>MCKDKNEKKNYEHVNANEKNGYLASEKNELTKNKVEEHTYDYDYVVIGGGPGGMASAKEAAAHGARVLLFDYVKPSSQGTKWGIGGTCVNVGCVPKKLMHYAGHMGSIFKLDSKAYGWKFDNLKHDWKKLVTTVQSHIRSLNFSYMTGLRSSKVKYINGLAKLKDKNTVSYYLKGDLSKEETVTGKYILIATGCRPHIPDDVEGAKELSITSDDIFSLKKDPGKTLVVGASYVALECSGFLNSLGYDVTVAVRSIVLRGFDQQCAVKVKLYMEEQGVMFKNGILPKKLTKMDDKILVEFSDKTSELYDTVLYAIGRKGDIDGLNLESLNMNVNKSNNKIIADHLSCTNIPSIFAVGDVAENVPELAPVAIKAGEILARRLFKDSDEIMDYSYIPTSIYTPIEYGACGYSEEKAYELYGKSNVEVFLQEFNNLEISAVHRQKHIRAQKDEYDLDVSSTCLAKLVCLKNEDNRVIGFHYVGPNAGEVTQGMALALRLKVKKKDFDNCIGIHPTDAESFMNLFVTISSGLSYAAKGGSGGGKCG[4x];>RGSHHHHHHGSVKIVTSQAEFDSIISQNELVIVDFFAEWCGPSKRIAPFYEECSK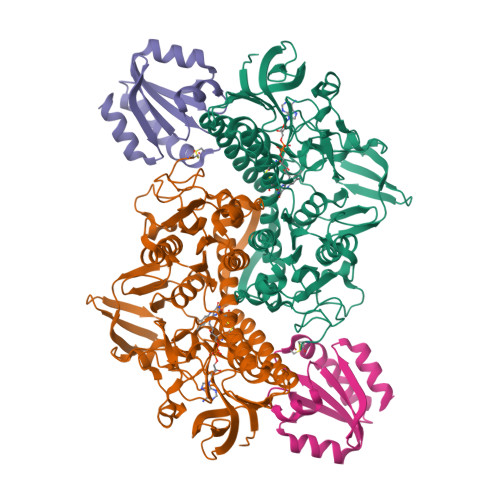TYTKMVFIKVDVDEVSEVTEKENITSMPTFKVYKNGSSVDTLLGANDSALKQLIEKYAA[4x]>[2x]MSRVLLCSAGHSSMVVPEAFHAVPEGFEEVHVFTTDSEKFNPVVLNDFFHSLPNVRFSITKCHGLADILNERDFEFYQEMLWQWYLTKMPDNELPYVCLSGGIKSMSASLQKAATLFGAQSVFHVLADNNPRNIEEMFDALQKGQIHFIEMGYEPGWAALRRLKKILPINEGCSRDNFKPLISKS

In order to identify novel CARF effectors, we used Foldseek18 to search for proteins with structural homology to CARF domain of the Cam1 effector. This method rendered a 600-residue protein containing an N-terminal CARF domain followed by a linker region and a C-terminal adenosine deaminase (ADA) domain, with accession number HAJ98955.1 from an unknown Bacteriodales bacterium (hereafter named CRISPR-associated deaminase, CRISPR-associated adenosine deaminase 1 [Cad1]), for which homologs were already identified in a previous bioinformatic screen. cad1 is located immediately downstream the cas10-csm genes of a type III-A CRISPR locus. Further analysis of cad1 homologs showed that over 70% associate in genomes containing type III systems (mostly belonging to the A and B subtypes) and exist within many unique phyla of bacteria. These data suggest that Cad1 is a widespread effector in type III CRISPR-Cas systems. Altogether, these data demonstrate that Cad1 deaminates ATP molecules to ITP through the formation of an hexameric complex that requires a Mg+2 or Mn+2 cofactor and an activating cA4 or cA6 ligand. While the triggering of a growth arrest in the host is a common strategy of all CARF effectors, we believe that Cad1 introduces a new mode of defense for CRISPR-Cas systems that couples nucleotide deamination activity to a sequence-specific, RNA-guided adaptive immune response.

To further test this finding, we purified a hexa-histidyl-tagged CARF domain (residues 1–185, Cad1-CARF-His6) and tested the binding of different cOAs using isothermal titration calorimetry (ITC). We found that Cad1-CARF-His6 binds to both cA6 and cA4 with a kD of 30 and 700 nM, respectively. We also co-crystallized cA6 and cA4 with Cad1-CARF-His6 and solved the crystal structures at 1.8 and 2.4 Å resolution, respectively. Although both cOA ligands were fully accommodated in the electropositive pocket of apo Cad1-CARF-His6, they affected differently the angle between the two C-terminal legs of the CARF monomers. While cA6 binding produced a minor change (from 58° in the apo structure to 55°), cA4 binding opened this angle to 76°, most likely a consequence of the deep burial of cA4 within the pocket. The Watson-Crick edges of several adenosines of bound cA6 and cA4 form intermolecular hydrogen bonds group of charged residues within the pocket, including K104, that account for the specificity of cOA recognition. We obtained a small but clear peak with the same retention time as cA6, a result that indicates that the hexameric form of the cyclic adenylate is the main ligand of Cad1 in staphylococci.>[2x]PFVNKQFNYKDPVNGVDIAYIKIPNAGQMQPVKAFKIHNKIWVIPERDTFTNPEEGDLNPPPEAKQVPVSYYDSTYLSTDNEKDNYLKGVTKLFERIYSTDLGRMLLTSIVRGIPFWGGSTIDTELKVIDTNCINVIQPDGSYRSEELNLVI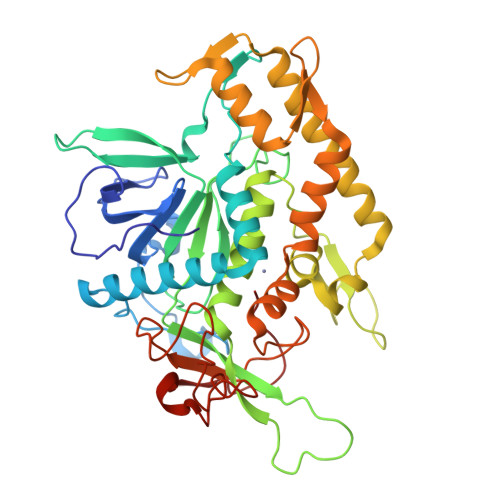IGPSADIIQFECKSFGHEVLNLTRNGYGSTQYIRFSPDFTFGFEESLEVDTNPLLGAGKFATDPAVTLAHQLIHAGHRLYGIAINPNRVFKVNTNAYYEMSGLEVSFEELRTFGGHDAKFIDSLQENEFRLYYYNKFKDIASTLNKAKSIVGTTASLQYMKNVFKEKYLLSEDTSGKFSVDKLKFDKLYKMLTEIYTEDNFVKFFKVLNRKTFLNFDKAVFKINIVPKVNYTIYDGFNLRNTNLAANFNGQNTEINNMNFTKLKNFTPGHHHHHH1H-isoindol-3-amine 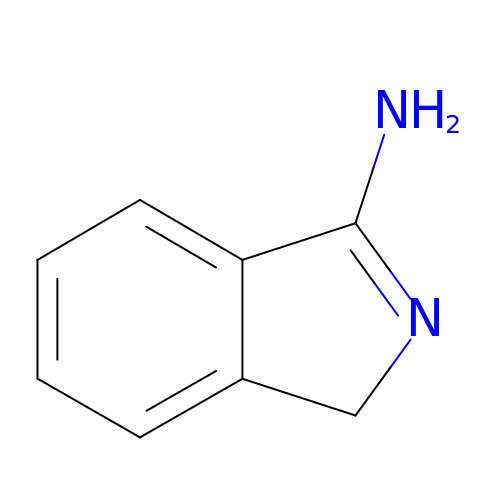| C8 H8 N2 | MTKKGHVQPVOXIL-UHFFFAOYSA-N> ETGVFQKAVDQSIEKKIVLRNGTEAFDSWEKPPLPVYTQFYFFNVTNPEEILRGETPRVEEVGPYTYRELRNKANIQFGDNGTTISAVSNKAYVFERDQSVGDPKIDLIRTLNIPVLTVIEWSQVHFLR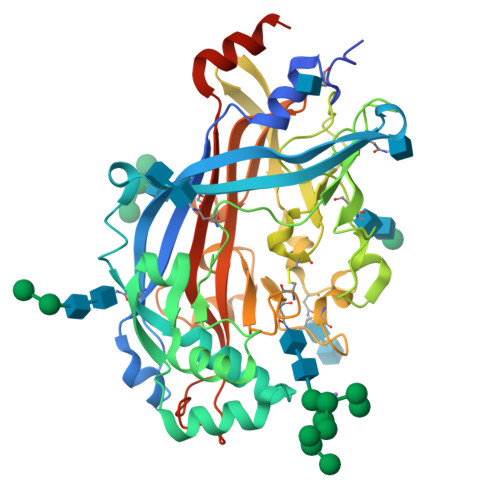EIIEAMLKAYQQKLFVTHTVDELLWGYKDEILSLIHVFRPDISPYFGLFYEKNGTNDGDYVFLTGEDSYLNFTKIVEWNGKTSLDWWITDKCNMINGTDGDSFHPLITKDEVLYVFPSDFCRSVYITFSDYESVQGLPAFRYKVPAEILANTSDNAGFCIPEGNCLGSGVLNVSICKNGAPIIMSFPHFYQADERFVSAIEGMHPNQEDHETFVDINPLTGIILKAAKRFQINIYVKKLDDFVETGDIRTMVFPVMYLNESVHIDKETASRLKSMINTGTKHHHHHH> AGVMTGAKFTQIQFGMTRQQVLDIAGAENCETGGSFGDSIHCRGHAAGDYYAYATFGFTSAAADAKVDSKSQEKLLAPSAPTLTLAKFNQVTVGMTRAQVLATVGQGSCTTWSEYYPAYPSTAGVTLSLSCFDVDGYSSTGF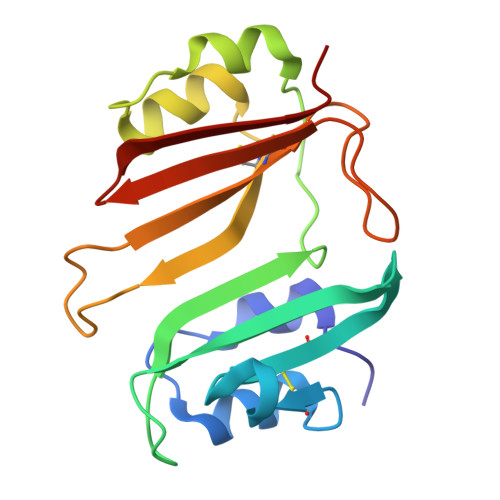YRGSAHLWFTDGVLQGKRQWDLV> TQVFDLEGYGAISRAMGGTSSSYYTGNAALISNPATLSFAPDGNQFELGLDVVTTDIKVHDSHGAEPKSSTYAVGAQLSYVAQLDDWRFGAGLFVSSLGTEYGSKSFLSQTENGIQTSFDNSSRLIVLRAPIGFSYQATSKLTFGASVDLVWTSLNLELLLPSSQVGALTAQGNLSGGLVPSLAGFVGTGGAAHFSLSRNSTAGGAVDAVGWGGRLGLTYKLTDNTVLGAMYNFKTSVGDLEGKATLSAISGDGAVLPLDGDIRVKNFEMPASLTLGLAHQFNERWVVAADIKRAYWGDVMDSMNVAFISQLGGIDVALPHRYQDITVASIGTAYKYNNDLTLRAGYSYAQQALDSELILPVIPAYLKRHVTFGGEYDFDKDSRINLAISFGLRERVQTPSYLAGTEMLRQSHSQINAVVSYSKNFHHHHHH

Thus far, only the FadL OM channel family has been shown to mediate transport of hydrophobics. PpF1 has three FadL orthologs, of which TodX (Pput_2883) and CymD (Pput_2901) are located in the adjacent tod and cym/cmt operons respectively. Here we show, by using an integrated approach combining growth assays, X-ray crystallography and molecular dynamics (MD) simulations, that MAH uptake as the first step in biodegradation does occur via lateral diffusion. In the presence of TodX/CymD, robust growth is observed, providing the first direct evidence for MAH transport by FadL-type channels.

The lateral opening in TodX involves both β-strand S2 and S3, contrasting with EcFadL in which only strand S3 is involved. Strand S2 in TodX bulges outward, whereas S3 has a less pronounced kink in the same place as EcFadL. To flatten the S2 bulge, we removed seven residues that were not visible in the density of TodX, replaced a proline with alanine and inserted an alanine to connect the strands (ΔS2). To flatten the S3 kink in the ΔS2 mutant, we removed the conserved glycine residue G104 to give ΔS2S3. We determined the X-ray crystal structures of both TodX variants which showed that, as expected, the size of the lateral opening is drastically reduced as a result of the flattening of the strands, while the remainder of the mutant structures are very similar to those of wild type. The two TodX mutant channels ΔS2 and ΔS2S3 have much smaller lateral openings, while retaining overall high structural similarity to the wild-type protein. Plate growth assays with vapour-phase toluene showed background growth for the TodX and CymD lateral opening mutants, indicating that they are defective in toluene uptake. For TodX, background growth is already observed for the ΔS2 mutant, so the effect of the additional flattening of strand S3 in the ΔS2S3 variant cannot be assessed.> DEHELLETA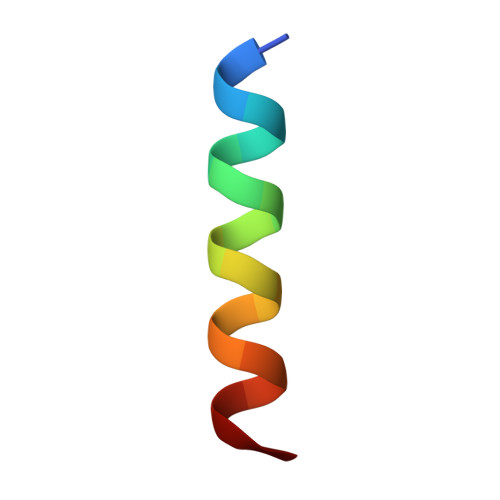ARWFYEIAKR>[4x]SAASNP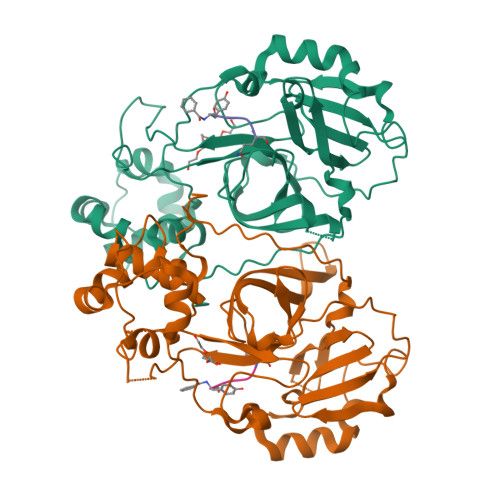SISHIVLEMPVAINPLIKYTTRTSVSSLRGAVVNGYIYIQRHLFGSKKQEFEACYNNGKGLLNCKNLERSKYDIDSAELIGTLIRIPLHDKHSIPHISIHPDPLSYNGPVTLYLSRYDTELNKDVLCVHTGFMSEGHHDIKTVFGDCGGMLFDPKGRLLGLHCAGSDDVVFMDTTTGKSNIWTSYKLQHPSEIMITLNNEINLPNPANYDFETTKVVYQHPLRNVCATLETLQHLTNKTNAKLPYDSRLLSDFNITAEQYNQYGYYIDYNNFVNNFNRYTTTTIGTKSFETCIKYGLMDNKKPDYYNQ;>XYYNQ[3x]> GMVSRSPFESFQWKSDIFNCESTDIDNFYLLLEQEMTRLGMVEKNLGEVGKYKVSLYQSPAAKSGLPSLLISAGFHGEESA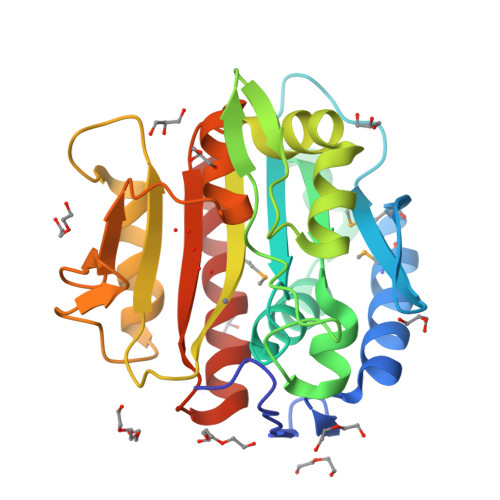GPWGLLHFLSEASADLFERVNLSLLPLVNPTGFSRGHRFNKYGENPNRGFVFENGKPKANEHTSVEGKLLLDHAQLLIAACRDGILTCHEDVLSREAYVYSFEPSQVPGRFSLDLRDTLGGYFPIAVDGEIDACPVKDGLIFNHFDTSFEACLVRSGARVGACTETPALQNFDQRVLANSAAMTHFLALCAPLCD> MSSLSRELVFLILQFLDEEKFKETVHKLEQESGFFFNMKYFEEKV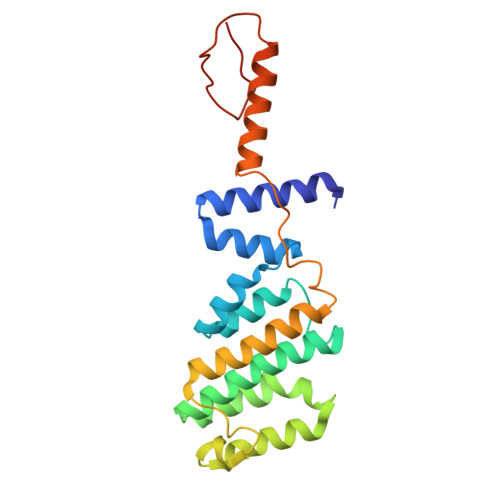HAGEWDEVEKYLSGFTKVDDNRYSMKIFFEIRKQKYLEALDRHDRAKAVDILVKDLKVFSTFNEELYKEITQLLTLENFRENEQLSKYGDTKSARSIMLIELKKLIEANPLFREKLVFPTLKASRLRTLINQSLNWQHQLCKNPRPNPDIKTLFTDHTCTPPNG> GSPQDLTVSLIPVSGLKAGKNAPSAKIAKLVVNSTTLKEFGVRGISNNVVDSTGTAWRVAGKNTGKEIGVGLSSDSLRRSDSTEKWNGVNWMTFNSNDTLDIVLTGPAQNVTADTYPITLDVVGYQP;> VNQQLNSATKLFSVKLGATRVIYHAGTAGATLSVSNPQNYPILVQSSVKAADKSSPAPFLVMPPLFRLEANQQSQLRIVRTGGDMPTDRETLQWVCIKAVPPENEPSDTQAKGATLDLNLSINACDKLIFRPDAVKGTPEDVAGNLRWVETGNKLKVENPTPFYMNLASVTVGGKPITGLEYVPPFADKTLNMPGSAHGDIEWRVIT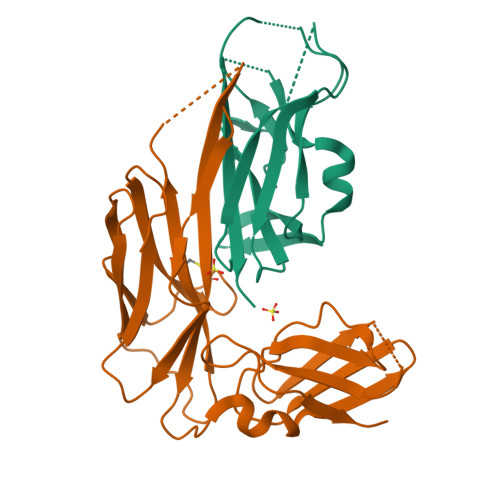DFGGESHPFHYVLK> SNAGGSSPITGLVYDQRMMLHHNMWDSHHPELPQRISRIFSRHEELRLLSRCHRIPARLATEEELALCHSSKHISIIKSSEHMKPRDLNRLGDEYNSIFISNESYTCALLAAGSCFNSAQAILTGQVRNAVAIVRPPGHHAEKDTACG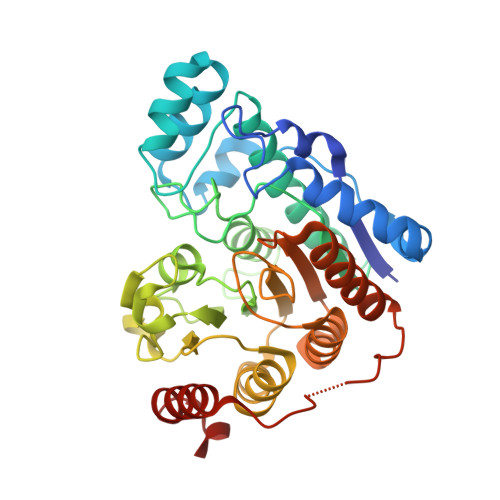FCFFNTAALTARYAQSITRESLRVLIVDWDVHHGNGTQHIFEEDDSVLYISLHRYEDGAFFPNSEDANYDKVGLGKGRGYNVNIPWNGGKMGDPEYMAAFHHLVMPIAREFAPELVLVSAGFDAARGDPLGGFQVTPEGYAHLTHQLMSLAAGRVLIILEGGFNLTSISESMSMCTSMLLGDSPPSLDHLTPLKTSATVSINNVLRAHAPFWSSLR> CDLPQTHNLRNKRALTLLVKMRRLSPLSCLKDRKDFG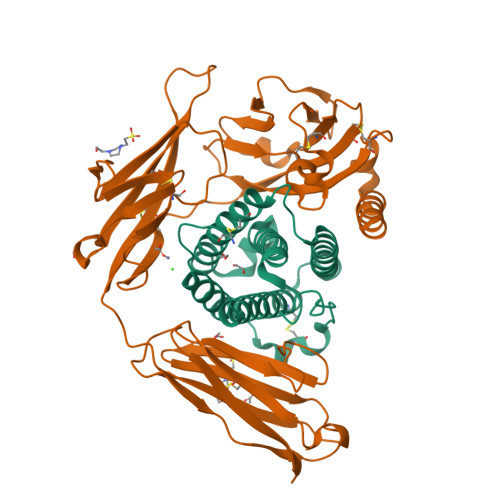FPQEKVGAQQIQEAQAIPVLSELTQQVLNIFTSKDSSAAWNATLLDSFCNEVHQQLNDLKACVMQQVGVQESPLTQEDSLLAVRKYFHRITVYLREKKHSPCAWEVVRAEVWRALSSSVNLLARLSKEE;> MIDIENEITEFFNKMRDTLPAKDSKWLNPSCMFGGTMNDMAALGEPFSAKCPPIEDSLLSHRYNDKDNVVNWEKIGKTRRPLNRRVKNGDLWIANYTSNDSHRRYLCTVTTKNGDCVQGIVRSHIRKPPSCIPETYELGTHDKYGIDLYCGILYAKHYNNITWYKNNQELIIDGTKYSQSGQNLIIHNPELEDSGRYDCYVHYDDVRIKNDIVVSRCKILTVIPSQDHRFKLILDPKINVTIGEPANITCTAVSTSLLVDDVLIDWENPSGWIIGLDFGVYSILTSSGGITEATLYFENVTEEYIGNTYTCRGHNYYFDKTLTTTVVLE> MSSTIFYRFKSQRNTSRILFDGTGLTVFDLKREIIQENKLGDGTDFQLKIYNPDTEEEYDDDAFVIPRSTSVIVKRSPAIKSFSVHSRLKGNVGAAALGNATRYVTGRPRVLQKRQHTATTTANV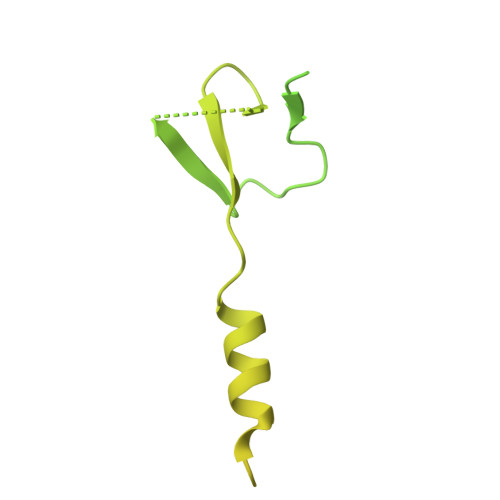SGTTEEERIASMFATQENQWEQTQEEMSAATPVFFKSQTNKNSAQENEGPPPPGYMCYRCGGRDHWIKNCPTNSDPNFEGKRIRRTTGIPKKFLKSIEIDPETMTPEEMAQRKIMITDEGKFVVQVEDKQSWEDYQRKRENRQIDGDETIWRKGHFKDLPDDLKCPLTGGLLRQPVKTSKCCNIDFSKEALENALVESDFVCPNCETRDILLDSLVPDQDKEKEVETFLKKQEELHGSSKDGNQPETKKMKLMDPTGTAGLNNNTSLPTSVNNGGTPVPPVPLPFGIPPFPMFPMPFMPPTATITNPHQADASPKK> SGGGGGILEKLGDICFSLRYVPTAGKLTVVILEAKNLKKMDVGGLSDPYVKIHLMQNGKRLKKKKTTIKKNTLNPYYNESFSFEVPFEQIQKVQVVVTVLDYDKIGKNDAIGKVFVGYNSTGAELRHWSDMLANPRRPIAQWHTLQVEEEV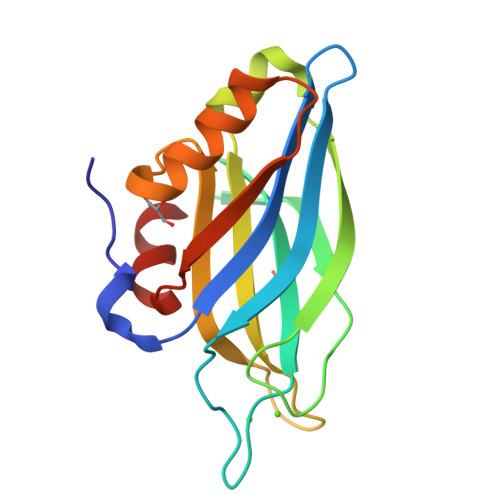DAMLAVKK> MADYKDDDDKSGPDEVDASGRVRKPVVSTISKGGYLQGNVNGRLPSLGNKEPPGQEKVQLKRKVTLLRGVSIIIGTIIGAGIFISPKGVLQNTGSVGMSLTIWTVCGVLSLFGALSYAELGTTIKKSGGHYTYILEVFGPLPAFVRVWVELLIIRPAATAVISLAFGRYILEPFFIQCEIPELAIKLITAVGITVVMVLNSMSVSWSARIQIFLTFCKLTAILIIIVPGVMQLIKGQTQNFKDAFSGRDSSITRLPLAFYYGMYAYAGWFYLNFVTEEVENPEKTIPLAICISMAIVTIGYVLTNVAYFTTINAEELLLSNAVAVTFSERLLGNFSLAVPIFVALSCFGSMNGGVFAVSRLFYVASREGHLPEILSMIHVRKHTPLPAVIVLHPLTMIMLFSGDLDSLLNFLSFARWLFIGLAVAGLIYLRYKCPDMHRPFKVPLFIPALFSFTCLFMVALSLYSDPFSTGIGFVITLTGVPAYYLFIIWDKKPRWFRIMSEKITRTLQIIL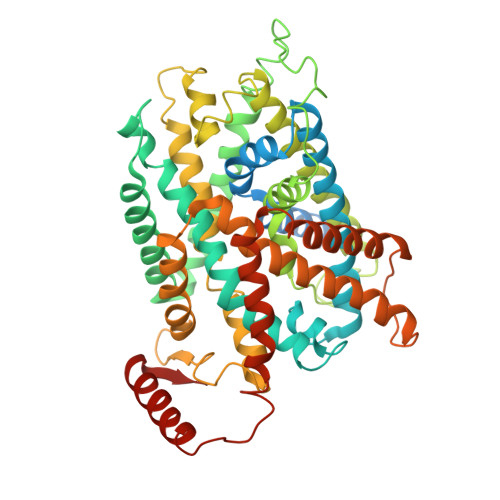EVVPEEDKL>MKMNQFINALMAKMTLDEKIGQLNLPGAGDITTGQASSSGIAQKIKEGKVGGLFNIKSVTKIKEVQRIAVEESRLKIPLLFGMDVIHGYETAFPIPLGLSCTWDMELIEKSARIAAIEASADGICWTFSPMVDISRDPRWGRVSEGSGEDPYLGAQIAKAMVKGYQGKDFSDNTSIMACVKHFALYGAGEAGRDYNTVDMSRVRMYNEYFPPYKAAVDAGVGSVMTSFNEIDGIPATGNKWLMTDVLRKRIGAFKGFVVTNYTAINEMIDHGMGDLQTVSALALRAGVDMDMVGEGFLTTLKKSLQEGKITQAQIDAACKRILEAKYKLGLFSDPYKYCNEERARTQIFTPEHRKIAREIAAQSFVLLKNDNNVLPLKKSGTIALVGPLADNRVNMPGTWSVAAKHAESVSLLEGLKKAAGNDARILYAHGSNLDEDKSLIERATMFGKTLKYDPRPKDVVIKEAVDIANQADVIVAALGESAEMSGEASSRSNIEIPALQRELLQALLKTGKPVVLVLFTGRPLALTWEHENVPAILNVWFAGTEAGDAISDALFGVVNPSGKLSATFPRNVGQVPIYYNHKNTGRPLPEGQWFQKFRSNYLDVPNDPLYPFGYGLSFTKFTYGDLKLSSTNLKGNQTLTASIELTNSGDYDGA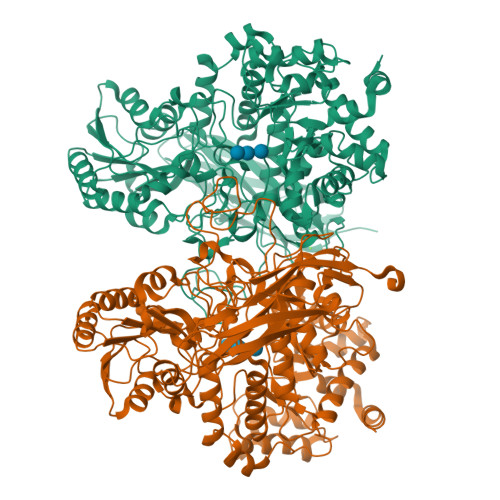EVVQLYIRDLVGSTTRPVKELKGFQKVFLKKGETKTITFKITPEDLKFYNYDLKYDWEPGEFVIMVGGNSRDLKSQKINWLKDPAFLYKVVINSKLEGKPIPNPLLGLDSTRTGHHHHHH[2x]>[2x]VVHGQTAKTITIK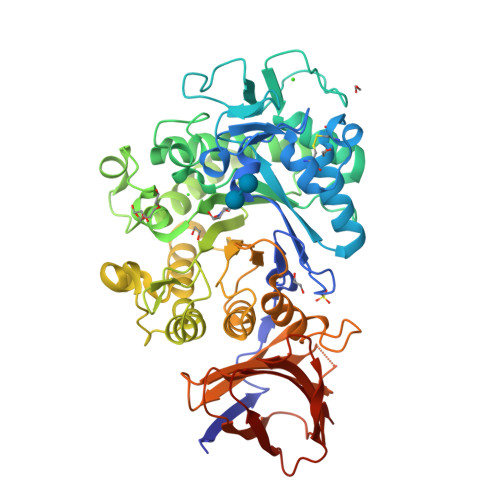VDTFKDRKPISPYIYGTNQDLAGDENMAARRLGGNRMTGYNWENNMSNAGSDWQHSSDNYLCSNGGLTQAECEKPGAVVTSFHDQSLKLGTYSLVTLPMAGYVAADGNGSVQESEAAPSARWNQVVNAKNAPFQLQPDLNDNYVYVDEFVHFLVNKYGTASTKAGVKGYALDNEPALWSHTHPRIHPEKVGAKELVDRSVSLSKAVKAIDAGAEVFGPVLYGFGAYKDLQTAPDWDSVKGNYSWFVDYYLDQMRLSSQVEGKRLLDVFDVHWYPEAMGGGIRITNEVGNDETKKARMQAPRTLWDPTYKEDSWIAQWFSEFLPILPRLKQSVDKYYPGTKLAMTSYSYGGENDISGGIAMTDVLGILGKNDVYMANYWKLKDGVNNYVSAAYKLYRNYDGKNSTFGDTSVSAQTSDIVNSSVHASVTNASDKELHLVVMNKSMDSAFDAQFDLSGAKTYISGKVWGFDKNSSQIKEAAPITQISGNRFTYTVPPLTAYHIVLTTGNYTSPV> TGMSREEVESLIQEVLEVYPEKARKDRNKHLAVNDPAVTQSKKCIISNKKSQPGLMTIRGCAYAGSKGVVWGPIKDMIHISHGPVGCGQYSRAGRRNYYIGTTGVNAFVTMNFTSDFQEKDIVFGGDKKLAKLIDEVETLFPL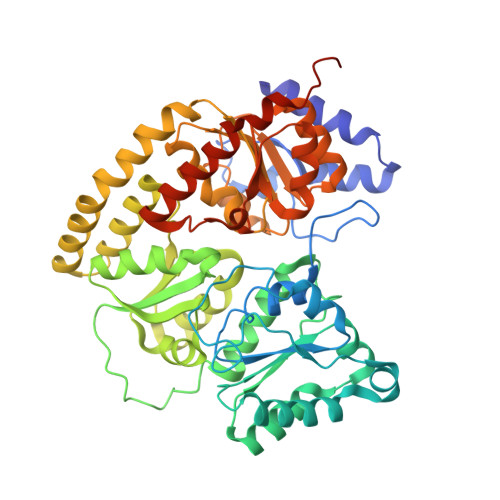NKGISVQSECPIGLIGDDIESVSKVKGAELSKTIVPVRCEGFRGVSQSLGHHIANDAVRDWVLGKRDEDTTFASTPYDVAIIGDYNIGGDAWSSRILLEEMGLRCVAQWSGDGSISEIELTPKVKLNLVHCYRSMNYISRHMEEKYGIPWMEYNFFGPTKTIESLRAIAAKFDESIQKKCEEVIAKYKPEWEAVVAKYRPRLEGKRVMLYIGGLRPRHVIGAYEDLGMEVVGTGYEFAHNDDYDRTMKEMGDSTLLYDDVTGYEFEEFVKRIKPDLIGSGIKEKFIFQKMGIPFREMHSWDYSGPYHGFDGFAIFARDMDMTLNNPCWKKLQAPWEASEGAEKVAASA> SSRPATARKSSGLSGTVRIPGDKSISHRSFMFGGLASGETRITGLLEGEDVINT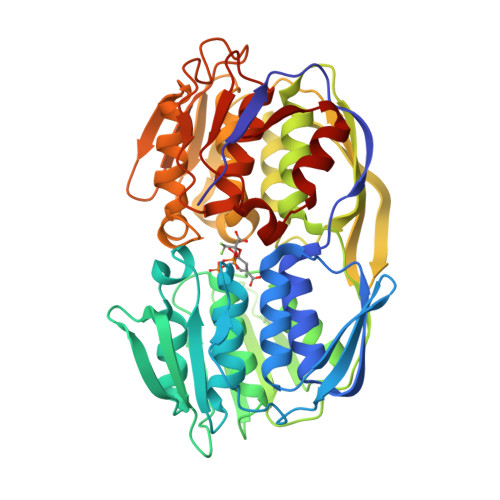GKAMQAMGARIRKEGDTWIIDGVGNGGLLAPEAPLDFGNAGTGCRLTMGLVGVYDFDSTFIGDASLTKRPMGRVLNPLREMGVQVKSEDGDRLPVTLRGPKTPTPITYRVPMASAQVKSAVLLAGLNTPGITTVIEPIMTRDHTEKMLQGFGANLTVETDADGVRTIRLEGRGKLTGQVIDVPGDPSSTAFPLVAALLVPGSDVTILNVLMNPTRTGLILTLQEMGADIEVINPRLAGGEDVADLRVRSSTLKGVTVPEDRAPSMIDEYPILAVAAAFAEGATVMNGLEELRVKESDRLSAVANGLKLNGVDCDEGETSLVVRGRPDGKGLGNASGAAVATHLDHRIAMSFLVMGLVSENPVTVDDATMIATSFPEFMDLMAGLGAKIELS>HHHHHHMSAIKPDMKINLRMEGNVNGHHFVIDGDGTGKPFEGKQSMDLEVKEGGPLPFAFDILTTAFHYGNRVFAEYPDHIQDYFKQSFPKGYSWERSLTFEDGGICIARNDITMEGDTFYNKVRFHGTNFPANGPVMQKKTLKWEPS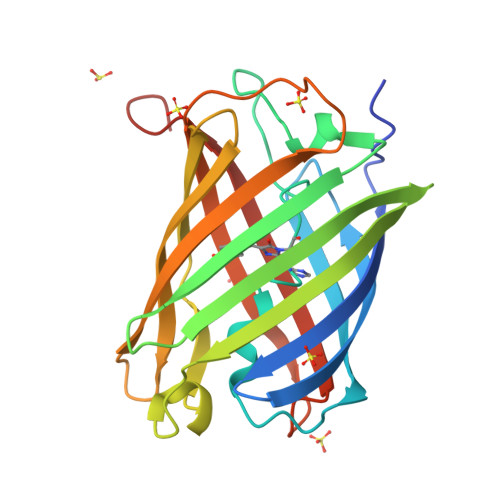TEKMYVRDGVLTGDIHMALLLEGNAHYRCDFRTTYKAKEKGVKLPGYHFVDHCIEILSHDKDYNKVKLYEHAVAHSGLPDNARR[4x]> KLPPGWEKRMSXGRVYYFNHI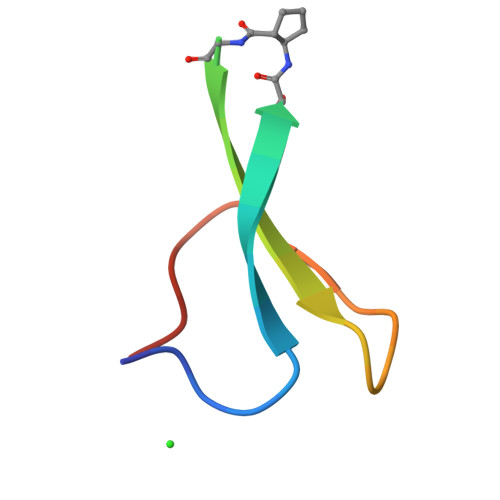TNASQWERPSG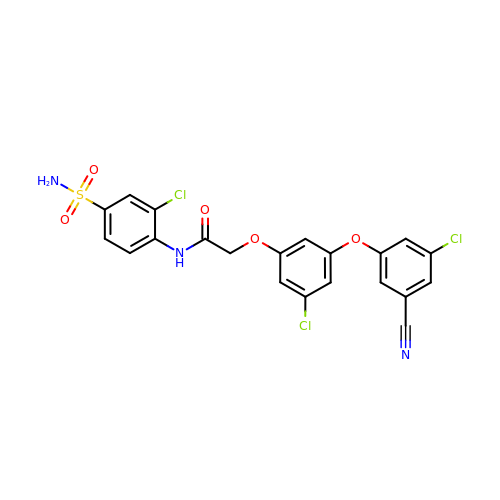2-[3-chloro-5-(3-chloro-5-cyanophenoxy)phenoxy]-N-(2-chloro-4-sulfamoylphenyl)acetamide | C21 H14 Cl3 N3 O5 S | GYBNBRVJAPRVLI-UHFFFAOYSA-N> VPSSALSEVSLR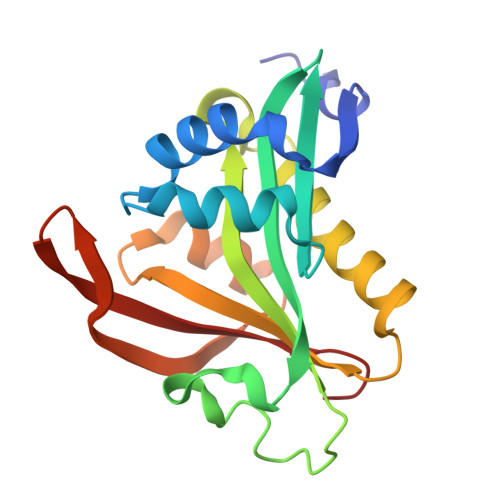LLCHDDIDTVKHLCGDWFPIEYPDSWYRDITSNKKFFSLAATYRGAIVGMIVAEIKNRTKIHKEDGDILASNFSVDTQVAYILSLGVVKEFRKHGIGSLLLESLKDHISTTAQDHCKAIYLHVLTTNNTAINFYENRDFKQHHYLPYYYSIRGVLKDGFTYVLYINGG> SNAMQSTSNHLWLLS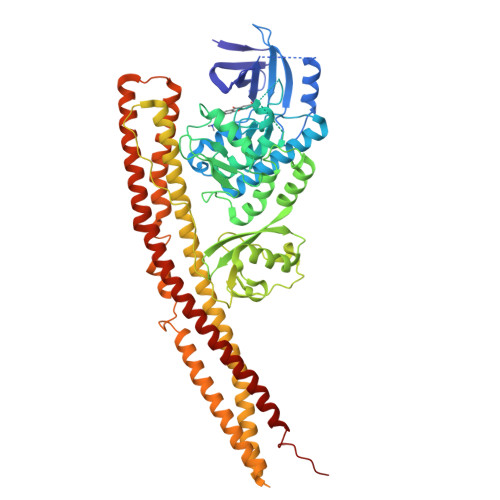DILGQGATANVFRGRHKKTGDLFAIKVFNNISFLRPVDVQMREFEVLKKLNHKNIVKLFAIEEETTTRHKVLIMEFCPCGSLYTVLEEPSNAYGLPESEFLIVLRDVVGGMNHLRENGIVHRDIKPGNIMRVIGEDGQSVYKLTDFGAARELEDDEQFVSLYGTEEYLHPDMYERAVLRKDHQKKYGATVDLWSIGVTFYHAATGSLPFRPFEGPRRNKEVMYKIITGKPSGAISGVQKAENGPIDWSGDMPVSCSLSRGLQVLLTPVLANILEADQEKCWGFDQFFAETSDILHRMVIHVFSLQQMTAHKIYIHSYNTATIFHELVYKQTKIISSNQELIYEGRRLVLEPGRLAQHFPKTTEENPIFVVSREPLNTIGLIYEKISLPKVHPRYDLDGDASMAKAITGVVCYACRIASTLLLYQELMRKGIRWLIELIKDDYNETVHKKTEVVITLDFCIRNIEKTVKVYEKLMKINLEAAELGEISDIHTKLLRLSSSQGTIETSLQDIDSRLSPGGSLADAWAHQEGTHPKDRNVEKLQVLLNCMTEIYYQFKKDKAERRLAYNEEQIHKFDKQKLYYHATKAMTHFTDECVKKYEAFLNKSEEWIRKMLHLRKQLLSLTNQCFDIEEEVSKYQEYTNELQET>[8x]SMALASKTAIVTGAARGIGFGIAQVLAREGARVIIADRDAHGEAAAASL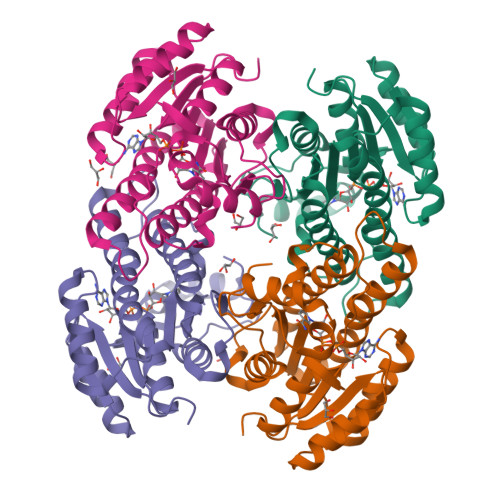RESGAQALFISCNIAEKTQVEALFSQAEEAFGPVDILVNNAGINRDAMLHKLTEADWDTVIDVNLKGTFLCMQQAAIRMRERGAGRIINIASASWLGNVGQTNYSASKAGVVGMTKTACRELAKKGVTVNAICPGFIDTDMTRGVPENVWQIMISKIPAGYAGEAKDVGECVAFLASDGARYINGEVINVGGGMVL dodecane-1,12-diamine | 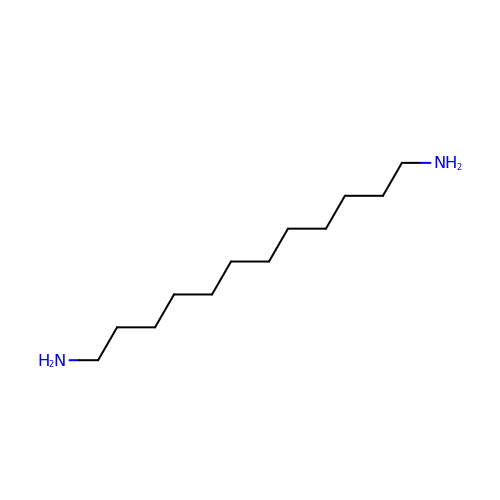C12 H28 N2 | QFTYSVGGYOXFRQ-UHFFFAOYSA-N> CKDKDLLKGLDQEQANEVIAVLQMHNIEANKIDSGKLGYSITVAEPDFTAAVYWIKTYQLPPRPRVEIAQMFPADSLVSSPRAEKARLYSAIEQRLEQSLQTMEGVLSARVHISYDIDAGENGRPPKPVHLSALAVYERGSPLAHQISDIKRFLKNSFADVDYDNISVVLSERSDAQLQAP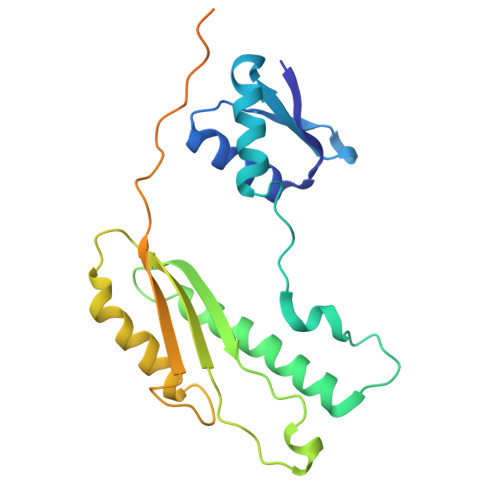GTPVKRNSFATSWIVLIILLSVMSAGFGVWYYKNHYARNKKGITADDKAKSSNE> RDPRDVP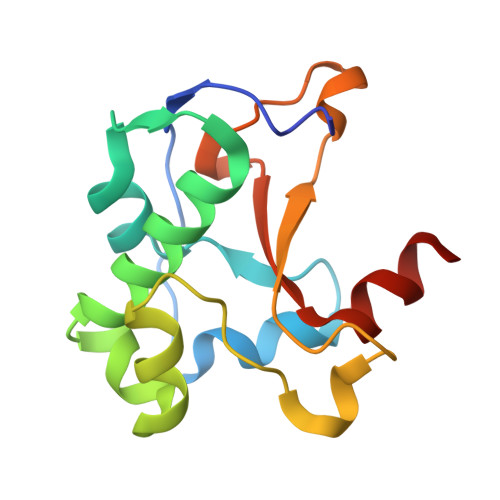GAATGKGQPVSGNWLGAASQGEGAPIPSQIADKLRGKTFKNWRDFREQFWIAVANDPELSKQFNPGSLAVMRDGGAPYVRESEQAGGRIKIEIHHKVRIADGGGVYNMGNLVAVTPKRHIEIHKGGK>[2x]GGCUCUGGAGAGAACC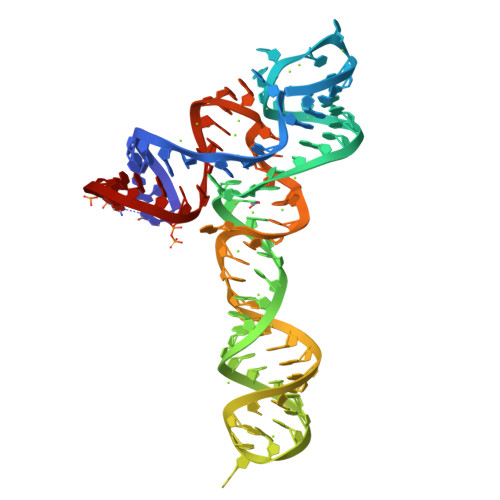GUUUAAUCGGUCGCCGAAGGAGCAAGCUCUGCGGAAACGCAGAGUGAAACUCUCAGGCAAAAGGACAGAGUC>SLFELGKMILQETGKNPAKSYGAYGCNCGVLGRGKPKDATDRCCYVHKCCYKKLTGCNPKKDRYSYSWKDKTIVCGENNPCLKELCECDKAVAICLRENLGTYNKKYRYHLKPFCKK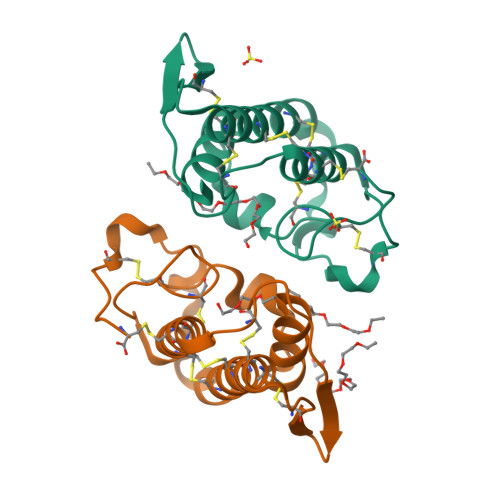ADPC[2x]> GAGCAGACTTG;> ACACCACTCA;> CATGT;> TCTGAGTGAGGTCTGC

In this work, we exhaustively probe the ability of all 36 immobile HJ sequences to form DNA crystals in two different designed systems. Three separate self-assembling DNA crystal systems are described in this report: the “4 × 5” and “4 × 6” designs (collectively referred to as the 4 × N systems), and a third construct with a “scrambled” sequence variant of the 4 × 6 lattices. Self-assembly was mediated by three constituent oligonucleotides: (S1) containing four sequence repeats of either 5 or 6 bases; (S2) composed of 21 bases containing complementary regions to both (S1); and (S3) which forms the second junction crossover. The HJ serves as the fundamental component at the core of each unit, and the ultimate assembly of the full lattice is facilitated by the complementary 2-base sticky ends that tail each duplex.

We hypothesized that it might be possible to introduce other unique immobile sequences that could provide slight perturbations in the junction angle, to potentially reduce the strain in the original system and yield a “relaxed,” periodic lattice. The 4 × 5 system robustly crystallized with 75% of the junctions, and we obtained crystals in all but 9 of 36 sequences. Of the resulting structures, 18 exhibited P32 symmetry with average cell dimensions a = b = 68.85 Å c = 60.09 Å, with only nine retaining the original P3221 symmetry with average cell edges a = b = 68.17 Å c = 60.60 Å. Although the cell parameters between the two symmetries were virtually indistinguishable, the differences between the periodicity of the lattices is dramatic, with vastly different cavity sizes. We hypothesize that even a small difference in junction angles could have a significant global effect on the assembly of the lattice, thereby eliminating the strain in the P3221 lattices.>[2x]DNSYKMDYPEMGLCIIINNKNFHKSTGMTSRSGTDVDAANLRETFRNLKYEVRNKNDL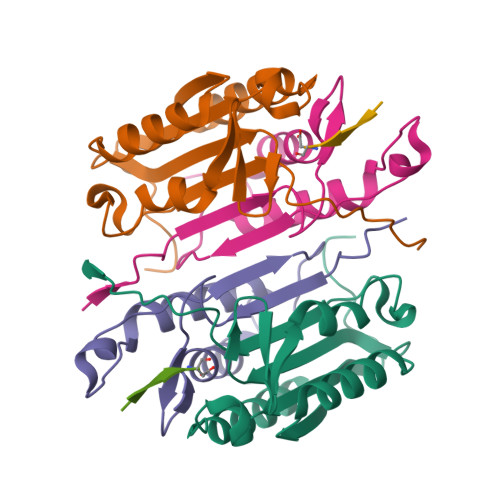TREEIVELMRDVSKEDHSKRSSFVCVLLSHGEEGIIFGTNGPVDLKKITNFFRGDRCRSLTGKPKLFIIQACRGTELDCGIET;>[2x]CHKIPVEADFLYAYSTAPGYYSWRNSKDGSWFIQSLCAMLKQYADKLEFMHILTRVNRKVATEFESFSFDATFHAKKQIPCIVSMLTKELYFYHH;>[2x]XVDVVD> MHNYVIIDAFASVPLEGNPVAVFFDADDLPPAQMQRIAREMNLSESTFVLKPRNGGDALIRIFTPVNELPFAGHPLLGTAIALGAHTDNHRLYLETQMGT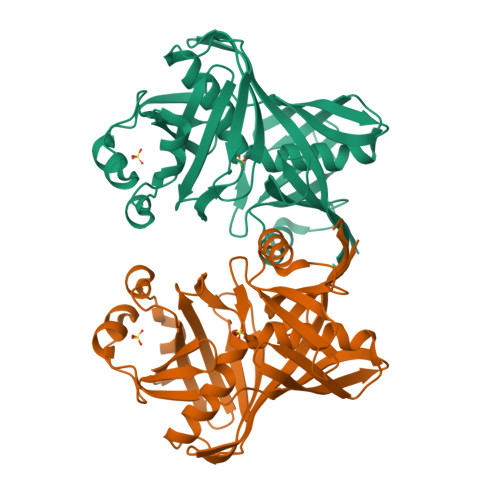IAFELERQNGSVIAASMDQPIPTWTALGRDAELLKALGISDSTFPIEIYHNGPRHVFVGLPSIDALSALHPDHRALSNFHDMAINCFAGAGRRWRSRMFSPAYGVVEDAATGSAAGPLAIHLARHGQIEFGQPVEILQGVEIGRPSLMFAKAEGRAEQLTRVEVSGNGVTFGRGTIVL> G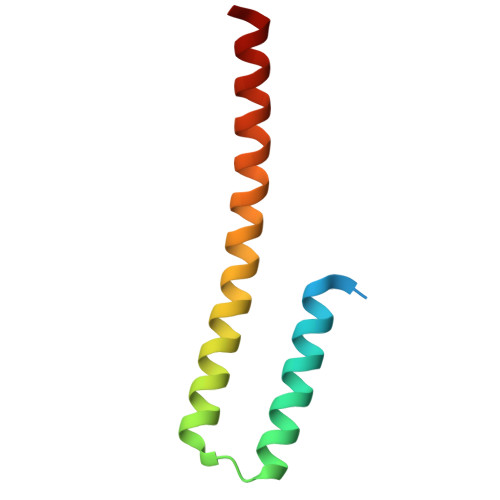SSLENLPPVAASIEQLLERQWSEGQQFLLEQGTPSDILGMLKSLHQLQVENRRLEEQIKNLTAKKERLQLLNAQLS>[3x]MHCKVSLLDDTVYECVVEKHAKGQDLLKRVCEHLNLLEEDYFGLAIWDNATSKTWLDSAKEIKKQVRGVPWNFTFNVKFYPPDPAQLTEDITRYYLCLQLRQDIVAGRLPCSFATLALLGSYTIQSELGDYDPELHGVDYVSDFKLAPNQTKELEEKVMELHKSYRSMTPAQADLEFLENAKKLSMYGVDLHKAKDLEGVDIILGVCSSGL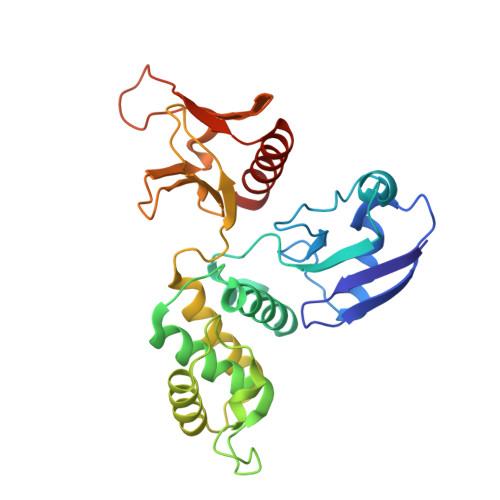LVYKDKLRINRFPWPKVLKISYKRSSFFIKIRPGEQEQYESTIGFKLPSYRAAKKLWKVCVEHHTFFR> IMPPEAEI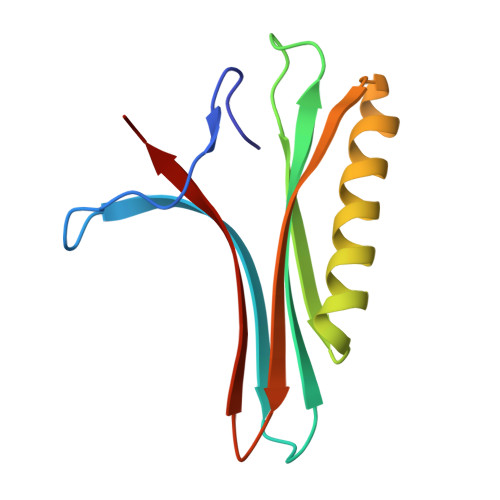VPLPKLPMGALVPTAYGYIISDVPGETISAAISVAIPKDKSLCGLIMEYEGKCSKKEAEKTVREMAKIGFEMRGWELDRIESIAVEHTVEKLGCAFAAAALWYK>[2x]MSEFSQTVPELVAWARKNDFSISLPVDRLSFLLAVATLNGERLDGEMSEGELVDAFRHVSDAFEQTSETIGVRANNAINDMVRQRLLNRFTSEQAEGNAIYRLTPLGIGITDY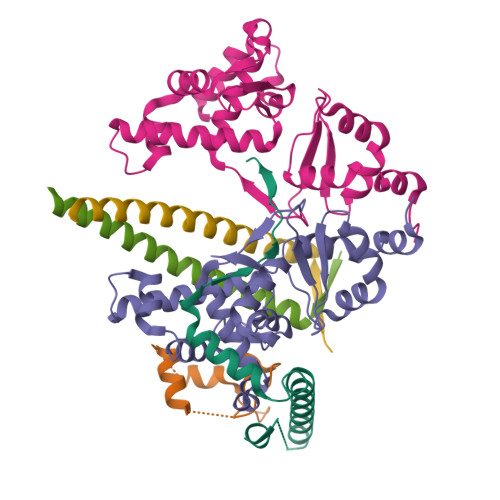YIRQREFSTLRLSMQLSIVAGELKRAADAAEEGGDEFHWHRNVYAPLKYSVAEIFDSIDLTQRLMDEQQQQVKDDIAQLLNKDWRAAISSCELLLSETSGTLRELQDTLEAAGDKLQANLLRIQDATMTHDDLHFVDRLVFDLQSKLDRIISWGQQSIDLWIGYDRHVHKFIRTAIDMDKNRVFAQRLRQSVQTYFDEPWALTYANADRLLDMRDEEMALRDEEVTGELPEDLEYEEFNEIREQLAAIIEEQLAVYKTRQVPLDLGLVVREYLSQYPRARHFDVARIVIDQAVRLGVAQADFTGLPAKWQPINDYGAKVQAHVIDKY;>[2x]MSSTNIEQVMPVKLAQALANPLFPALDSALRSGRHIGLDELDNHAFLMDFQEYLEEFYARYNVELIRAPEGFFYLRPRSTTLIPRSVLSELDMMVGKILCYLYLSPERLANEGIFTQQELYDELLTLADEAKLLKLVNNRSTGSDVDRQKLQEKVRSSLNRLRRLGMVWFMGHDSSKFRITESVFRFGADVRAGDDPREAQRRLIRDGEAMPIENHLQLNDETEENQPDSGEEE;>GPGMSRDLVTIPRDVWNDIQGYIDSLERENDSLKNQLMEADEYVAELEEKLNGTS[2x]> DEFQWKGLPVVKSGLDVGGMPTGTRYHRSPAWPEEQPGETHAPAPFGSGDKRYTFSQTEMLVNGLKPYTEPTAGVPPQLLSRAVTHVRSYIETIIGTHRSPVLTYHQACELLERTTSCGPFVQGLKGDYWDEEQQQYTGVLANHLEQAWDKANKGIAPRNAYKLALKDELRPIEKNKAGKRRLLWGCDAATTLIATAAFKAVATRLQVVTPMTPVAVGINMDSVQMQVMNDSLKGGVLYCLDYSKWDSTQNPAVTAASLAILERFAEPHPIVSCAIEALSSPAEGYVNDIKFVTRGGLPSGMPFTSVVNSINHMIYVAAAILQAYESHNVPYTGNVFQVETIHTYGGGCMYSVCPATASIFHTV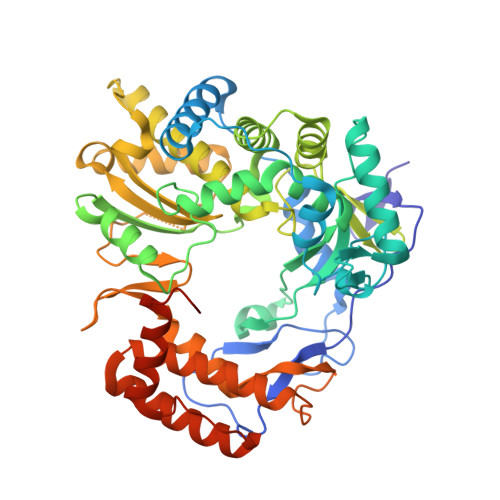LANLTSYGLKPTAADKSDAIKPTNTPVFLKRTFTQTPHGIRALLDITSITRQFYWLKANRTSDPSSPPAFDRQARSAQLENALAYASQHGPVMFDTVRQIAIKTAQGEGLVLVNTNYDQALATYNAWFIGGTVPDPVGHTEGTHKIVFEME> SMVEISALPLRDLDYIKLATDQFGCRFLQKKLETPSESNMVRDLMYEQIKPFFLDLILDPFGNYLVQKLCDYLTAEQKTLLIQTIYPNVFQISINQYGTRSLQKIIDTVDNEVQIDLIIKGFSQEFTSIEQVVTLINDLNGNHVIQKCIFKFSPSKFGFIIDAIVEQNNIITISTHKHGCCVLQKLLSVCTLQQIFKISVKIVQFLPGLINDQFGNYIIQFLLDIKELDFYLLAELFNRLSNELCQLSCLKFSSNVVEKFIKKLFRIITGFIVNNNGGA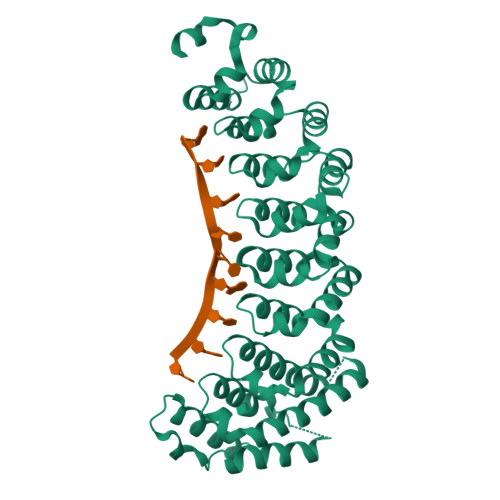SQRTAVASDDVINASMNILLTTIDIFTVNLNVLIRDNFGNYALQTLLDVKNYSPLLAYNKNSNAIGQNSSSTLNYGNFCNDFSLKIGNLIVLTKELLPSIKTTSYAKKIKLKVKAYAEATG>MRGSHHHHHHGSIEGRMEKINYLLPEESAEMTLNQVKSLRQIEGRLRKLFSLKNYQEVMPPSFEYTQLYTALESNGKTFNQEKMFQFIKHEGQSITLRYDFTLPLVRLYSQIKDSTSARYSYFGKIFRKEKRHKGRSTENYQIGIELFGESADKSELEILSLALQVIEQLGL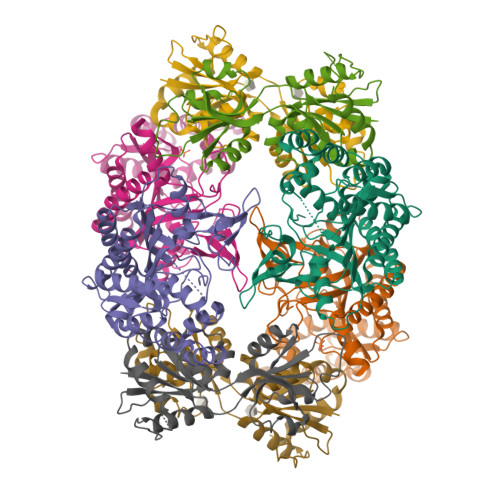NKTVFEIGSAKFFQRLCQLADGSTELLTELLLKKDLSGLNAFIEKNNFSKELRGLLKEIFITNELSRLENLVTNTKDDVLISSFDQLKEFSEKLSMIKPIIIDLGMVPKMDYYTDLMFKAYSSAANQPILSGGRYDQLLSNFQEEAFAIGFCCHMDTILKALERQELEEDND[4x];>MIKIAITKGRIQKQVTKLLENADYDVEPILNLGRELQIKTKDDLQIIFGKPNDVITFLEHGIVDIGFVGKDTLDENDFDDYYELLYLKIGQCIFALASYPDFSNKNFQRHKRIASKYPRVTKKYFAQKQEDIEIIKLEGSVELGPVVGLADAIVDIVETGNTLSANGLEVIEKISDISTRMIVNKSSFKFKKDKIIEMVERLEDAQTN[4x]>[2x]MSLAPYRVDFILLEHFSMASFTVAMDVLVTANLLRADSFQFTPLSLDGDRVLSDLGLELVATELSAAALKELDLLVVCGGLRTPLKYPELDRLLNDC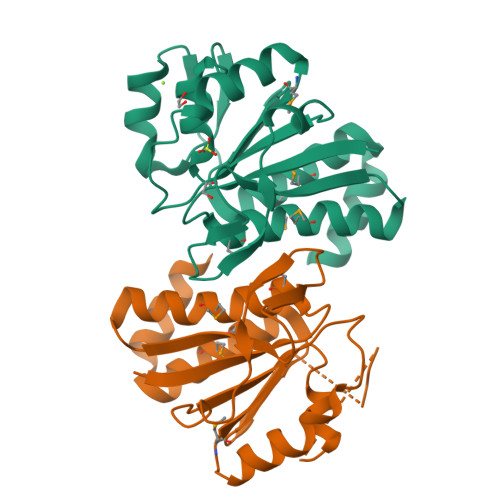AAHGMALGGLWNGAWFLGRAGVLDDYGCSIHPEQRASLSERSPQTRITPASFTLDRDRLSAASPNGAMELMLGLVRRLYGDGLAEGVEEILSFSGAREGHHHHHH5'-azido-8-[(2-{[2-(3-bromophenyl)ethyl]amino}-2-oxoethyl)sulfanyl]-5'-deoxyadenosine 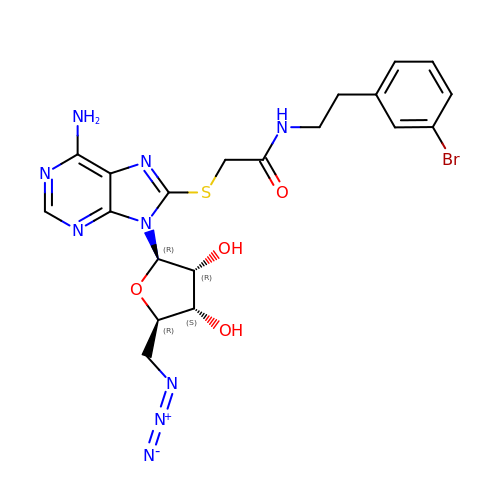| C20 H22 Br N9 O4 S | JYGMOYIMZQWVHO-BGIGGGFGSA-N>[2x]MSLTGNAQAATIADPSTLVVDTVGPVLTIGLNRPKKRNALNDGLMAALKDCLTDIPDQIRAVVIHGIGDHFSAGLDL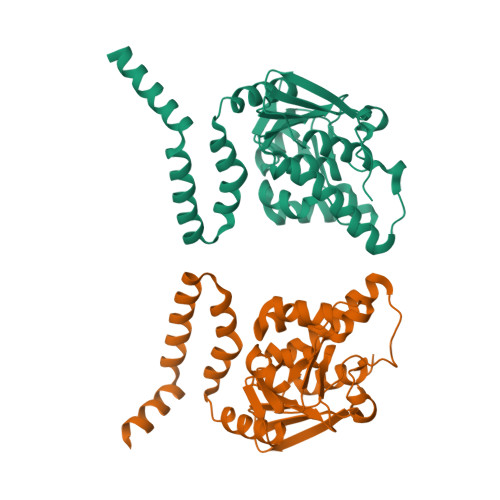SELRERDATEGLVHSQTWHRVFDKIQYCRVPVIAALKGAVIGGGLELACAAHIRVAEASAYYALPEGSRGIFVGGGGSVRLPRLIGVARMADMMLTGRVYSAAEGVVHGFSQYLIENGSAYDKALELGNRVAQNAPLTNFAVLQALPMIAEANPQTGLLMESLMATVAQSDQEAKTRIRAFLDHKTAKVREGHHHHHH>SLAALKSELQALKKEGFSPEELAALESELQALEKKLAALKSKLQALKG[2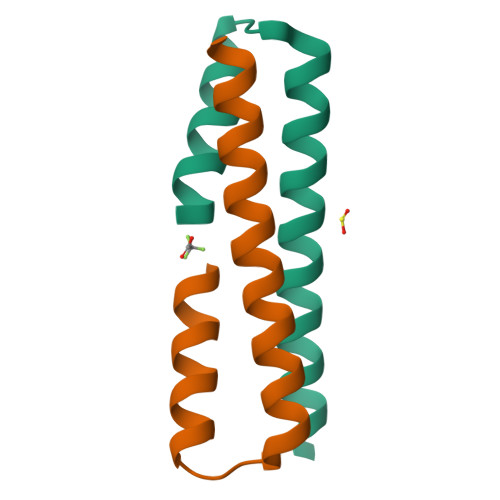x]> DYKDDDDKAAAQSLEFNSPADNYTVCEGDNATLSCFIDEHVTRVAWLNRSNILYAGNDRWTSDPRVRLLINTPEEFSILITEVGLGDEGLYTCSFQTRHQPYTTQVY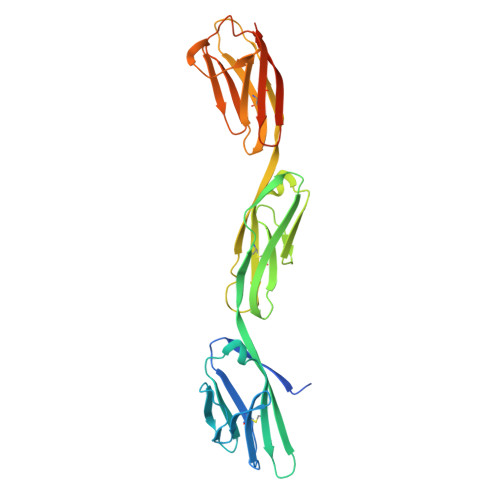LIVHVPARIVNISSPVTVNEGGNVNLLCLAVGRPEPTVTWRQLRDGFTSEGEILEISDIQRGQAGEYECVTHNGVNSAPDSRRVLVTVNYPPTITDVTSARTALGRAALLRCEAMAVPPADFQWYKDDRLLSSGTAEGLKVQTERTRSMLLFANVSARHYGNYTCRAANRLGASSASMRLLRPGSLENSALEVLFQ>MAGNSIGQLFRVTTCGESHGVGLMAIVDGVPPGLALTEEDLQKDLDRRKPGTSKFATQRKEPDQVEIISGVFEGKTTGTPIGLLIRNTDQKSKDYGNIAQTFRPGHADYTYTQKYGFRDYRGGGRSSARETAMRVAAGAIAKKYLAEKFGVLIRGHVTQIGNEVAEKLDWNEVPNNPFFC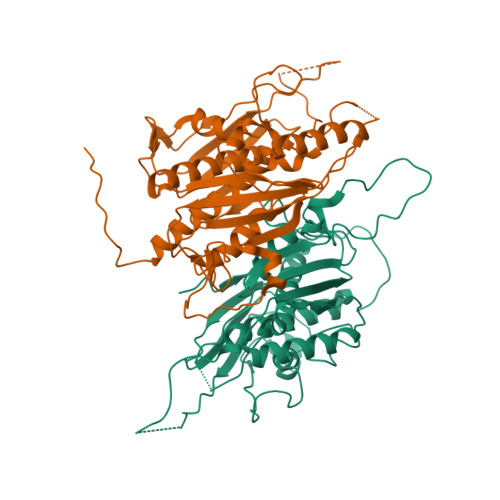GDVDAVPRFEALVTSLREQGTSCGAKLEILAEKVPVGWGEPVFDRLDADIAHAMMSINAVKGVEIGDGFAVAGQFGHETRDELTSHGFLANHAGGILGGISSGQTIRVAIALKPTASITTPGKTINLNREDTDVLTKGRHDPCVGVRATPIAEAMLAIVLMDHFLRHRAQNADVVPPFAPIEP[2x]>[2x]MSPFPLTSMDKAFITVLEMTPVLGTEIINYRDGMGRVLAQDVYAKDNLPPFPASVKD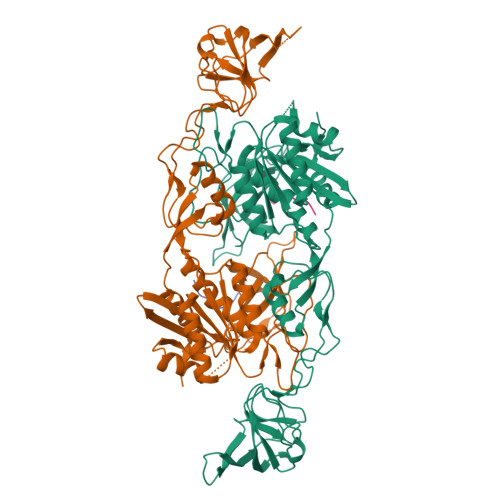GYAVRAADGPGDRFIIGESQAGEQPTQTVMPGQVMRVTTGAPIPCGADAVVQVEDTELIRESDDGTEELEVRILVQARPGQDIRPIGHDIKRGECVLAKGTHMGPSEIGLLATVGVTEVEVNKFPVVAVMSTGNELLNPEDDLLPGKIRDSNRSTLLATIQEHGYPTINLGIVGDNPDDLLNALNEGISRADVIITSGGVSMGEKDYLKQVLDIDLHAQIHFGRVFMKPGLPTTFATLDIDGVRKIIFALPGNPVSAVVTCNLFVVPALRKMQGILDPRPTIIKARLSCDVKLDPRPEYHRCILTWHHQEPLPWAQSTGNQMSSRLMSMRSANGLLMLPPKTEQYVELHKGEVVDVMVIGRL;>[2x]FSIVGTLYPIN CLC-2 is a voltage-gated chloride channel that contributes to electrical excitability and ion homeostasis in many different tissues. Among the nine mammalian CLC homologs, CLC-2 is uniquely activated by hyperpolarization, rather than depolarization, of the plasma membrane. The TM region of CLC-2 displays a typical CLC family symmetric homodimeric structure, with each subunit containing an independent Cl− pathway. All eukaryotic CLCs contain a pair of ‘cystathionine β-synthase’ (CBS) domains in their intracellular C-terminal domain (CTD).

We determined the structure of CLC-2 in complex with AK-42. The overall density for CLC2-TM-AK42 is very similar to that observed in apo CLC-2, but with an extra density that fits very well to the AK-42 molecule. Located at the extracellular side of Cl− pathway, the bound AK-42 appears to directly block Cl− permeation. In the binding site, AK-42’s phenyl ring nestles into a hydrophobic pocket lined by F306, F463, F459, M460, and L524. The carboxyl group of AK-42 forms hydrogen bonds with the side chain of S392 and backbone of K394. A third hydrogen bond – between K204 and the pyridine nitrogen of AK-42 – also contributes to AK-42’s stability in the binding pocket. The exception is residue M460, which moves ~3 Å to avoid a clash with AK-42’s phenyl ring. Notably, density corresponding to the N-terminal hairpin structure is not seen in the AK-42-bound structure. Intriguingly, the lack of density for the hairpin peptide in the AK-42-bound structure suggests that hairpin and AK-42 binding may be mutually exclusive.

>[2x]GEDWIFLVLLGLLMALVSWVMDYAIAACLQAQQWMSRGLNTSILLQYLAWVTYPVVLITFSAGFTQILAPQAVGSGIPEMKTILRGVVLKEYLTLKTFIAKVIGLTCALGSGMPLGKEGPFVHIASMCAALLSKFLSLFGGIYENESRNTEMLAAACAVGVGCCFAAPIGGVLFSIEVTSTFFAVRNYWRGFFAATFSAFIFRVLAVWNRDEETITALFKTRFRLDFPFDLQELPAFAVIGIASGFGGALFVYLNRKIVQVMRKQKTINRFLMRKRLLFPALVTLLISTLTFPPGFGQFMAGQLSQKETLVTLFDNRTWVRQGLVEELEPPSTSQAWNPPRANVFLTLVIFILMKFWMSALATTIPVPCGAFMPVFVIGAAFGRLVGESMAAWFPDGIHTDSSTYRIVPGGYAVVGAAALAGAVTHTVSTAVIVFELTGQIAHILPVMIAVILANAVAQSLQPSLYDSIIRIKKLPYLP>MGSSHHHHHHSSGLVPRGSMNQNLLVTKRDGSTERINLDKIHRVLDWAAEGLHNVSISQVELRSHIQFYDGIKTSDIHETIIKAAADLISRDAPDYQYLAARLAIFHLRKKAYGQFEPPALYDHVVKMVEMGKYDNHLLEDYTEEEFKQMDTFIDHDRDMTFSYAAVKQLEGKYLVQNRVTGEIYESAQFLYILVAACLFSNYPRETRLQYVKRFYDAVSTFKISLPTPIMSGVRTPTRQFSSCVLIECGDSLDSINATSSAIVKYVSQRAGIGINAGRIRALGSPIRGGEAFHTGCIPFYKHFQTAVKSCSQGGVRGGAATLFYPMWHLEVESLLVLKNNRGVEGNRVRHMDYGVQINKLMYTRLLKGEDITLFSPSDVPGLYDAFFADQEEFERLYTKYEKDDSIRKQRVKAVELFSLMMQERASTGRIYIQNVDHCNTHSPFDPAIAPVRQSNLCLEIALPTKPLNDVNDENGEIALCTLSAFNLGAINNLDELEELAILAVRALDALLDYQDYPIPAAKRGAMGRRTLGIGVINFAYYLAKHGKRYSDGSANNLTHKTFEAIQYYLLKASNELAKEQGACPWFNETTYAKGILPIDTYKKDLDTIANEPLHYDWEALRESIKTHGLRNSTLSALMPSETSSQISNATNGIEPPRGYVSIKASKDGILRQVVPDYEHLHDAYELLWEMPGNDGYLQLVGIMQKFIDQSISANTNYDPSRFPSGKVPMQQLLKDLLTAYKFGVKTLYYQNTRDGAEDAQDDLVPSIQDDGSDNVQVAPQEVEVSSYLVGQIDSEVDTDDLSNFQL[2x]

Class Ia ribonucleotide reductases (RNRs) are allosterically regulated by ATP and dATP to maintain the appropriate deoxyribonucleotide levels inside the cell for DNA biosynthesis and repair. The α2 subunit houses the active site and the allosteric sites, and the β2 subunit houses the di-iron-tyrosyl radical cofactor.3−6 On every round of turnover, these subunits come together to form an active α2β2 complex, which allows for the transfer of the radical species from β to α, affording ribonucleoside diphosphate reduction. Excess dATP inhibits RNR through the creation of an α–β interface that restricts the ability of β2 to obtain a position that is capable of radical transfer. ATP breaks the α–β interface, freeing β2 and restoring enzyme activity.

We, therefore, sought a different crystal form for α2 in which the β-hairpin region of the cone domain is less restricted by lattice contacts. With this in mind, we were able to obtain a new crystal form of α2 by fusing the 35 C-terminal residues of β (341–375) to the C terminus of an 8-residue truncated α (α2–βC35). The overall structure of this crystal form with dATP bound at 2.10-Å resolution is essentially identical to that observed above for free α2; however, the cone domain is slightly less restricted by lattice contacts near the β-hairpin. With the restraints of the crystal lattice relaxed, helix 2 adopts the unwound conformation, as in the α4β4 complex. The hydrophobic pocket vacated by H46 is left unfilled in this structure, and residues 19–27 (helix 1) and 35–43 (helix 2) that interact with β2 in the α4β4 complex are exposed to solvent. This structure thus demonstrates that specific contacts with β2 are not required for helix 2 to be unwound and this structure reveals a connection between dATP binding in site 1 and helix 2 unwinding.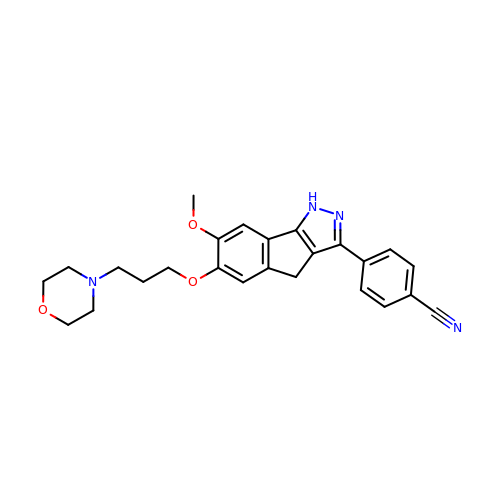4-{7-methoxy-6-[3-(morpholin-4-yl)propoxy]-1,4-dihydroindeno[1,2-c]pyrazol-3-yl}benzonitrile | C25 H26 N4 O3 | VSCASMLRSQQEQP-UHFFFAOYSA-N(10S)-3,3-dimethyl-8-{[(2S)-2-(phenoxymethyl)pyrrolidin-1-yl]sulfonyl}-2,3,4,10-tetrahydropyrimido[1,2-a]indol-10-ol 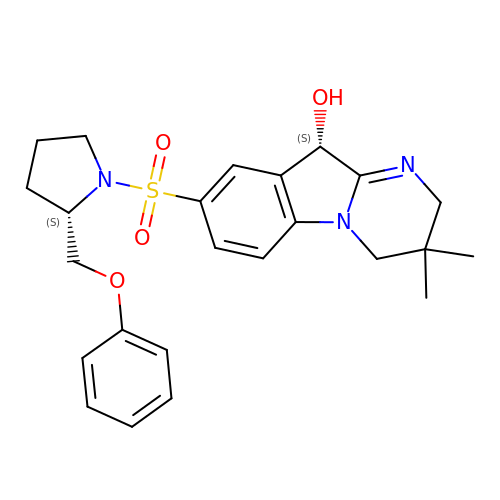| C24 H29 N3 O4 S | RPXBZVLBDLIKLZ-JTSKRJEESA-N>MSEDLRVGLFPVRYLVGTGLPGAPQLVLDLMVDTVDHSVVGRAAVSQAVSPPLNFHADVWGSYVFRLGPPPRRDGSGAIVQISLQGNQGGPQSNSMITFYGELLLKGDGKTGVASYRYYSNGSWHEVENVPVKADPELVPIEPGPVIGQSSMSAIGSAAMYGVAIQSAAASGDLAHMRTLSAYARQQLESRDEIAAALSEL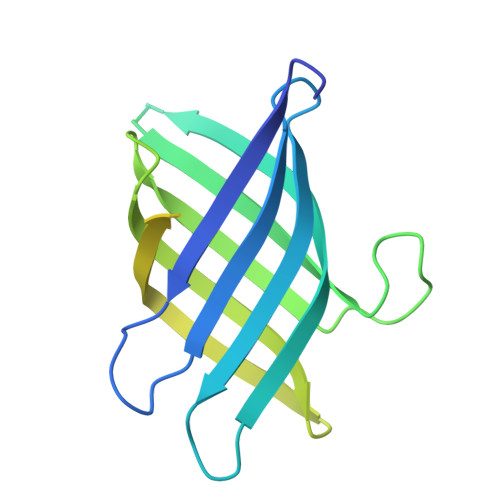KAEIAKLESRQHHHHHH[2x]4-(6-{[(1R)-1-(hydroxymethyl)propyl]amino}imidazo[1,2-b]pyridazin-3-yl)benzoic 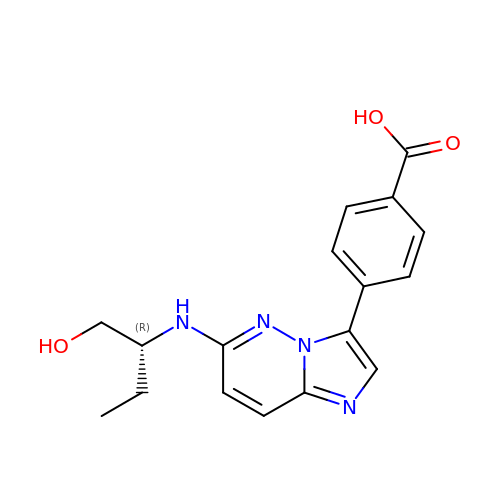acid | C17 H18 N4 O3 | KKZYGUVAFJCULH-CYBMUJFWSA-N S. cerevisiae, a genetically well-described system, harbors in its genome an endogenous virus known as L-A virus, a member of the Totivirus family, and its discovery was the main starting point of research on yeast virology. The L-A virus contains a single 4.6 kb double-stranded RNA (dsRNA), encoding for a capsid protein (Gag), and the viral RNA-dependent RNA polymerase fusion protein (Gag/Pol).

To derive solid molecular insights into the L-A virus structure within the cell extract, we acquired an additional cryo-EM dataset at 0.93 Å. A high-quality de novo model was built in the derived 3.21 Å L-A virus cryo-EM map (FSC = 0.143). The backbone was explicitly traceable; the α-helical pitch and β-strand separation were both discernable. Side chain densities were clearly visible, which allows us for the unambiguous placement of most side chains. The icosahedral protein shell has a triangulation number T = 1 organization, consisting of 60 structural units, with each unit comprising two chemically identical capsid proteins, formed by 120 protomers, with overall diameter (400 Å) and thickness (46 Å) comparable to its crystallographic counterpart. A similar opening diameter (18 Å) at the icosahedral fivefold axes was observed that is hypothesized to serve as a gate for the exit of viral mRNA and entry of nucleotide triphosphates. Detailed analysis of the L-A virus identified previously undescribed stabilizing cation-π interactions in the capsid that mediate interactions within and also across L-A protomers. In the asymmetric unit, 26 side chains are involved in forming 11 distinct cation-π interaction networks, formed within monomeric and dimeric interfaces (examples are shown in Fig. 2c). Structural changes compared to the crystal structure are detected in both capsomere subunits, specifically in loop regions (R94–V104; Y528–K536, G601–H607) of protomers A and B, respectively. Specifically, the flexible region spanning residues 528–534 encircles the active site. This loop element undergoes dynamic changes as it was not Cα-traceable in the cryo-EM map; however, in the crystal structure it was resolved, pointing to a regulatory role in the binding site accessibility.

>MLRFVTKNSQDKSSDLFSICSDRGTFVAHNRVRTDFKFDNLVFNRVYGVSQKFTLVGNPTVCFNEGSSYLEGIAKKYLTLDGGLAIDNVLNELRSTCGIPGNAVASHAYNITSWRWYDNHVALLMNMLRAYHLQVLTEQGQYSAGDIPMYHDGHVKIKLPVTIDDTAGPTQFAWPSDRSTDSYPDWAQFSESFPSIDVPYLDVRPLTVTEVNFVLMMMSKWHRRTNLAIDYEAPQLADKFAYRHALTVQDADEWIEGDRTDDQFRPPSSKVMLSALRKYVNHNRLYNQFYTAAQLLAQIMMKPVPNCAEGYAWLMHDALVNIPKFGSIRGRYPFLLSGDAALIQATALEDWSAIMAKPELVFTYAMQVSVALNTGLYLRRVKKTGFGTTIDDSYEDGAFLQPETFVQAALACCTGQDAPLNGMSDVYVTYPDLLEFDAVTQVPITVIEPAGYNIVDDHLVVVGVPVACSPYMIFPVAAFDTANPYCGNFVIKAANKYLRKGAVYDKLEAWKLAWALRVAGYDTHFKVYGDTHGLTKFYADNGDTWTHIPEFVTDGDVMEVFVTAIERRARHFVELPRLNSPAFFRSVEVSTTIYDTHVQAGAHAVYHASRINLDYVKPVSTGIQVINAGELKNYWGSVRRTQQGLGVVGLTMPAVMPTGEPTAGAAHEELIEQADNVLVE[2x]> MRGTRKYQHVIETPDPGKWELAGYEESLPISEKSNPMTRELDKADPSQLVQLLRDCDAEIFQEEDENLIHYHRLYSESVLKTMGDVAKRVQEVLKNPDDSLVVLSGCGTSGRLALLLANSFNGLLKGLHKTPCYCYIMSGGDRSIVTSQESSEDNPQLGAQELEKVCEGKKNVLFIGISCGLSAPFIAGQLDFCMRHLDVYLPVLVGFNPVSMARNERIEGWHSSFRQVAERLQTLHDSQKGFILNPAVGPEGVSGSSRMKGGSATKILLETLLLVAHKAESNVPVTEKCLLEILRTYERAHKVTYS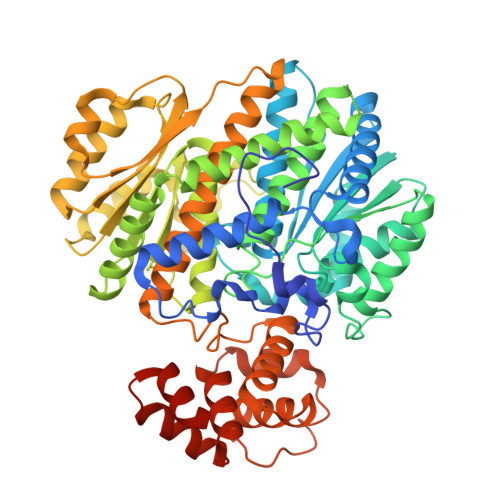QSKKIAALMKQTATSLQKKGHLYILGWGTLGLVGIMDAVECVPTYQADWRDVRGFITGGYHSIENKEGDLSSLGPQFSISHEDFVKNVLPSVSETDTVLLIFTLDDDLNQIEKLVALVKEKTSNIQVICHATAGQYLPNSLKKTIPSIIGLTWPILFLEYEGAFIQKFQRELSTKWILDTVTSGAYTLRGKIFRNFMVDFKINNSKLFHRATSVLQRLTGQSQQRCTEVLLQSIYGEQTLSEQIRNTTIAGHVEAAASQDKVLPVAIVSLLRSCTIQDSRSRINSSLSIRSAIESSMNVPGRKRGAEDSESR>GFDYDVVVVGGGFAGATAARECGLQGYRTLLLEARSRLGGRTFTSRFAGQEIELGGTWVHWLQPHVWAEMQRYGLGVVEDPLTNLDKTLIMYNDGIVESISPDEFGKNIRIAFEKLCHDAWEVFPRPHEPMFTERARELDKSSVLDRIKTLGLSRLQQAQINSYMALYAGETTDKFGLPGVLKLFACGGWNYDAFMDTETHYRIQGGTIGLINAMLTDSGAEVRMSVPVTAVEQVNGGVKIKTDDDEIITAGVVVMTVPLNTYKHIDFTPALSKGKQRFIKEGQLSKGAKLYVHVKQNLGRVFAFADEQQPLNWVQTRDYSDELGTILSITIARKETIDVNDRDAVTREVQKMFPGVEVLGTAAYDWTADPFSLGAWAAYGVGQLSRLKDLQAAEGRIVFAGAETSNGWHASIDGAVESGLRAGREVKQLLS[2x]

Nicotine oxidoreductase (NicA2) is a flavin-dependent enzyme that catalyzes the degradation of nicotine into the non-psychoactive metabolite N-methylmyosmine (NMM). NicA2 acts by degrading nicotine in the bloodstream before it reaches the brain. Clinical use of NicA2 is limited by its poor catalytic activity in the absence of its natural electron acceptor CycN. The higher in vivo activity of NicA2 is due to the presence of a cytochrome c, termed CycN, that acts as an alternative electron acceptor to O29.

We were unable to solve structures of NicA2 v320 but were fortunate to obtain well-diffracting crystals of NicA2 v321 in both the ligand-free and NMM-bound forms. The ligand-free structures of the wild-type and v321 enzymes are somewhat different, with the crystallized conformation of ligand-free v321 closely mimicking the NMM-bound state of both wild-type and variant enzymes. Analyzing differences in deuterium uptake between wild-type NicA2 and v321, we observed an increase in deuterium incorporation in NicA2 v321 compared to wild-type in both the ligand-free and NMM-bound states. Increased uptake is observed in the area surrounding the putative tunnel in v321, suggesting that it is more accessible to solvent. This is consistent with our hypothesis that mutations in this region facilitate O2 transport to the active site. The 19F spectrum of NicA2 v321 was strikingly different and was composed of a broad upfield-shifted major peak at −60.2 ppm and three highly overlapping downfield minor peaks. In summary, the 19F NMR spectra of the two ligand-free NicA2 molecules demonstrate a higher degree of conformational heterogeneity in the proposed oxygen tunnel in NicA3 v321 than in the wild-type protein. We observe that compared to the wild type, NicA2 v321 appears to have greater exposure to solvent in a mutation-rich region encompassing a putative O2 tunnel. This tunnel is also more conformationally heterogenous in the ligand-free condition of v321 than it is in the wild type. NicA2 v321 is active in vivo at a tenfold higher efficacy than wild-type NicA2 and can maintain blood nicotine concentrations at undetectable levels.>[2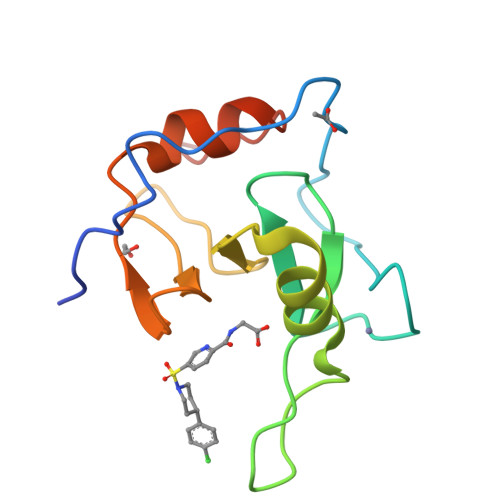x]GGEVRQVSKHAFSLKQLDNPARIPPCGWKCSKCDMRENLWLNLTDGSILCGRRYFDGSGGNNHAVEHYRETGYPLAVKLGTITPDGADVYSYDEDDMVLDPSLAEHLSHFGIDMLKMQKTD>AENLPNIVILATGGTIAGSAAANTQTTGYKAGALGVETLIQAVPELKTLANIKGEQVASIGSENMTSDVLLTLSKRVNELLARSDVDGVVITHGTDTLDESPYFLNLTVKSDKPVVFVAAMRPATAISADGPMNLYGAVKVAADKNSRGRGVLVVLNDRIGSARFISKTNASTLDTFKAPEEGYLGVIIGDKIYYQTRLDKVHTTRSVFDVTNVDKLPAVDIIYGYQDDPEYMYDASIKHGVKGIVYAGMGAGSVSKRGDAGIRKAESKG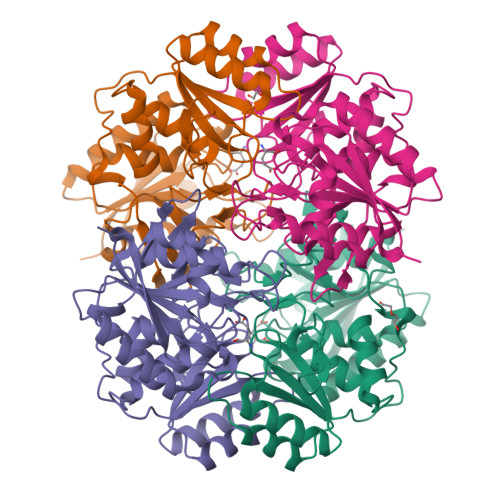IVVVRSSRTGSGIVPPDAGQPGLVADSLSPAKSRILLMLALTKTTNPAVIQDYFHAY[12x]>GGGGTGGGAGGAGGGT[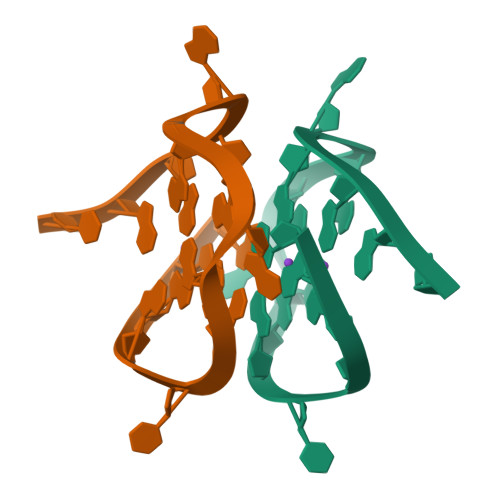4x]>[4x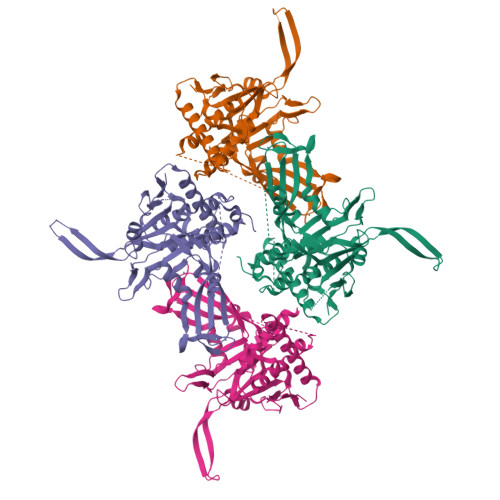]GRPPKGFVGLKNAGATCYMNSVIQQLYMIPSIRNGILAIEGTGSDVDDDMSGDEKQDNESNVDPRDDVFGYPQQFEDKPALSKTEDRAAYNIGVLRHLQVIFGHLAASRLQYYVPRGFWKQFRLWGEPVNLREQHDALEFFNSLVDSLDEALKALGHPAMLSKVLGGSFADQKICQGCPHRYECEESFTTLNVDIRNHQNLLDSLEQYVKGDLLEGANAYHCEKCNKKVDTVKRLLIKKLPPVLAIQLKRFDYDWERECAIKFNDYFEFPRELDMEPYTVAGVAKLEGDNVNPESQLIQQSEQSESETAGSTKYRLVGVLVHSGQASGGHYYSYIIQRNGGDGERNRWYKFDDGDVTECKMDDDEEMKNQCFGGEYMGEVFDHMMKRMSYRRQKRWWNAYILFYERMDTIDQDDELIRYIS>[2x]KFTEIFPVEDANYPYSAFIASVRKDVIKHCTDHKGIFQPVLPPEKKVPELWLYTELKTRTSSITLAIRMDNLYLVGFRTPGGVWWEFGKDGDTHLLGDNPRWLGFGGRYQDLIGNKGLETVTMGRAEMTRAVNDLAKKKKMATLEEEEVQMQMQMPEAADLA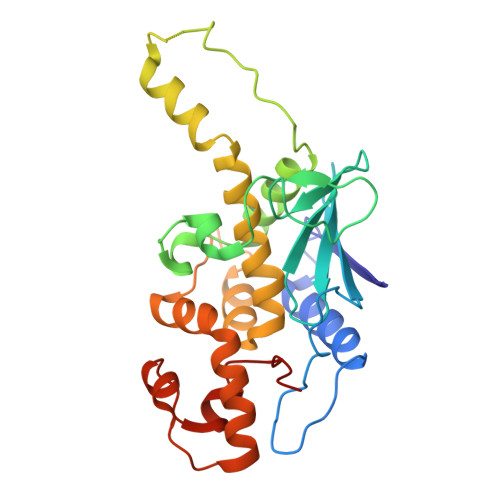AAAAADPQADTKSKLVKLVVMVCEGLRFNTVSRTVDAGFNSQHGVTLTVTQGKQVQKWDRISKAAFEWADHPTAVIPDMQKLGIKDKNEAARIVALVKNQTTA>[2x]AEIYNKDGNKVDLYGKAVGLHYFSKGNGENSYGGNGDMTYARLGF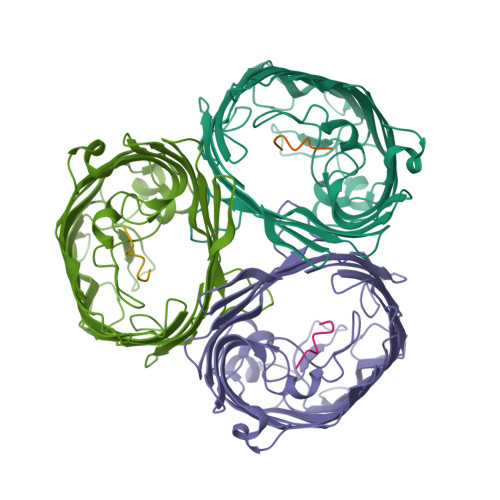KGETQINSDLTGYGQWEYNFQGNNSEGADAQTGNKTRLAFAGLKYADVGSFDYGRNYGVVYDALGYTDMLPEFGGDTAYSDDFFVGRVGGVATYRNSNFFGLVDGLNFAVQYLGKNERDTARRSNGDGVGGSISYEYEGFGIVGAYGAADRTNLQEAQPLGNGKKAEQWATGLKYDANNIYLAANYGETRNATPITNKFTNTSGFANKTQDVLLVAQYQFDFGLRPSIAYTKSKAKDVEGIGDVDLVNYFEVGATYYFNKNMSTYVDYIINQIDSDNKLGVGSDDTVAVGIVYQF> MEFFGESWKKHLSGEFGKPYFIKLMGFVAEERKHYTVYPPPHQVFTWTQMCDIKDVK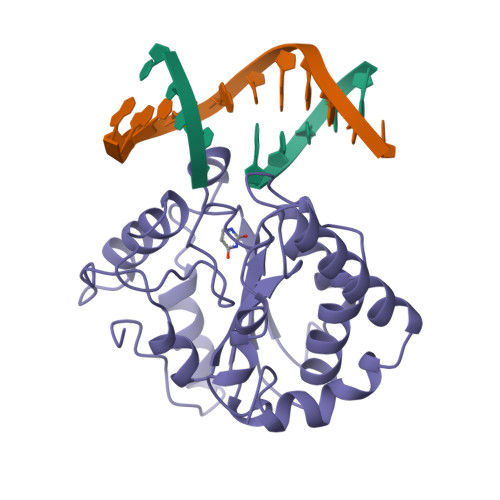VVILGQDPYHGPNQAHGLCFSVQRPVPPPPSLENIYKELSTDIEDFVHPGHGDLSGWAKQGVLLLNAVLTVRAHQANSHKERGWEQFTDAVVSWLNQNSNGLVFLLWGSYAQKKGSAIDRKRHHVLQTAHPSPLSVYRGFFGCRHFSKTNELLQKSGKKPIDWKEL>MEAPASYVEPYLGDAIVGNRRPAVRLTLDLLDHRVPEADIVEDLLAAAQREVGERWYRNELSPADEHLASGVAGAALDALAAELPPPTRDGLVVVACAEGDWHSLSAQMFGETLRASGFDVSVLGASTPRTAVVDFLTRAGGDSLAVSCNMPIFFPGVAQLINAAHEIGVPVIVGGRAFGDDDRRAARLGADAWAAGASEAAEILAGWHARRPEVGSEPAPLDGAALRLFAASSTLATATVDELTASSSPILDLDADQVDQLREHLVFAVQFLAAARLVDDDSIFEDFLVWIDELLRTRDVPREVLAAGLEGLRAKVIAVDPGATRLLDAAWSSQPVEVADGDGLEHHHHHH[2x]

Here we identify and characterise a sub-family of multi-centre photoreceptors, termed photocobilins, that use B12 and biliverdin (BV) to sense light across the visible spectrum. We have identified and characterised two types of photocobilins, one from Saccharothrix syringae (SasPcob) that represents a standalone photocobilin photoreceptor and a more complex protein that consists of a photocobilin diguanylate cyclase (DGC) fusion from Acidimicrobiaceae bacterium (AbDPcob) that is representative of a photocobilin domain fused to an enzyme domain. Crystal structures reveal close juxtaposition of the B12 and BV chromophores, an arrangement that facilitates optical coupling. Light-triggered conversion of the B12 affects quaternary structure, in turn leading to light-activation of associated enzyme domains.

Despite the low sequence identity (~34%), the structures of the two photocobilin proteins are similar, with an RMSD value of 1.63 Å for 464 C-alphas after structural alignment. Both the SasPcob and AbPcob proteins contain the W-(10)x-EH and E/DxH motifs in the B12-binding domain, which is found in other light dependent CarH-like B12 photoreceptors. The D ring is positioned out of the ABC plane by approximately 40° due to close interactions with Trp296. Although the putative BV binding globin scaffold is retained in AbPcob, the reduced BV affinity is most likely due to replacement of a key BV binding residue, Asp270 in SasPcob, with a His (Fig. 5f−i). The crystal structure of AbPcob revealed that steric hindrance by this His residue interferes with BV binding, unlike in SasPcob. Molecular dynamics simulations and ligand docking demonstrate that rearrangement of surrounding residues could allow BV to bind with AbPcob in certain conformations, where hydrophobic interactions with residues in the binding pocket (e.g., Leu252, Trp289, Leu294, Arg297, Val299 and Val303) contribute to retain BV in the correct orientation (Fig. 6c−h). The lack of the main binding interaction with the Asp residue in AbPcob may explain the absence of any obvious spectral shift and increase in absorbance at 700 nm upon BV binding that is observed for SasPcob. These findings could explain the lower BV occupancy levels for AbPcob whilst retaining the ability to respond to red light. Unfortunately, we were unable to obtain crystals of the full length AbDPcob protein or the light state of AbPcob. The weaker binding and lower occupancy levels (~20%) of BV in AbDPcob suggest that evolutionary pressures may have reduced the requirement for BV and resulted in a different role for the globin-like domain in these more complex fusion proteins.>[2x]GSSHHHHHHSQDPNSSSTK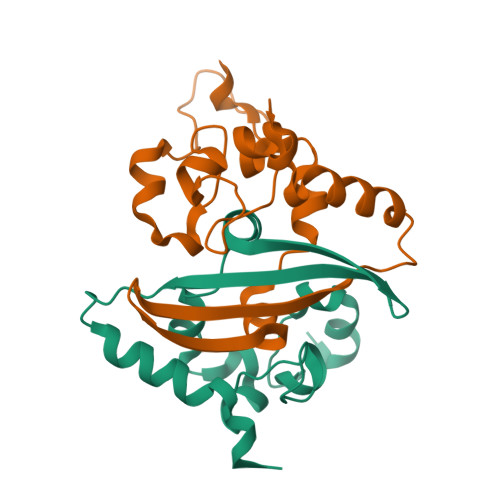KSAAEASKKPRQKRTATKAYNVTQAFGRRGPEQTQGNFGDQELIRQGTDYKHWPQIAQFAPSASAFFGMSRIGMEVTPSGTWLTYTGAIKLDDKDPNFKDQVILLNKHIDAYKTFP> MSGALNQLVAVGKQDAFITGDNLDNSVWRNVTKKVSNFAMESIENYINVNPGSTTSIVVGRFGDLVRKVTLEITMKKGSTTNPFYPSEQYVKYAHLSIGGQIVYRIDDFPTWTRVHEELFMD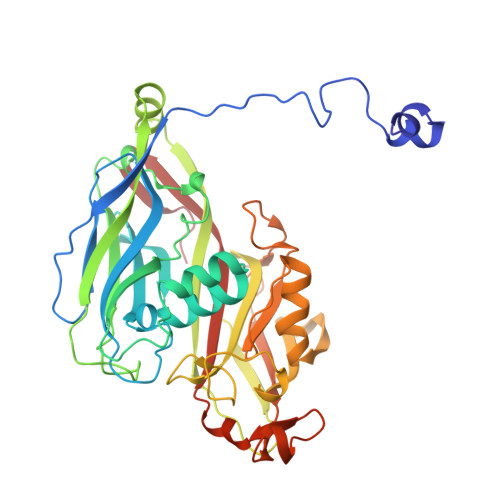PDTRATNQRVNNFRPEDPVGAIRKFYLDIPLFFTDDASKALPLIALQYHEVKLDVLFASPGDIPGIDASYTPTVECYIDYVFLDTPEREWFARNTHMYVIEQLQHYNNVFSVAAVEQTKRLNLPFTMPTRYLIWLLKTGADGVYTTSGYPFENNDSYAAIKSAKLQFNGTDRFSERPGYYFTTVQPQDAFGRSPSAGIYVYSFGLDVTGMTSKGALNFSRMDNATLSITTKAATAATISDVYNQSTTLASAITDFTSIAIYAKSFNVLKIDYGMGGMLFAN> MNQNGDKNEGKLFQLPSLPPWKTPRFNKANFNNFTTPLRKRSTRVINDDSMPITGEVLEERTADDLYGINMDVDE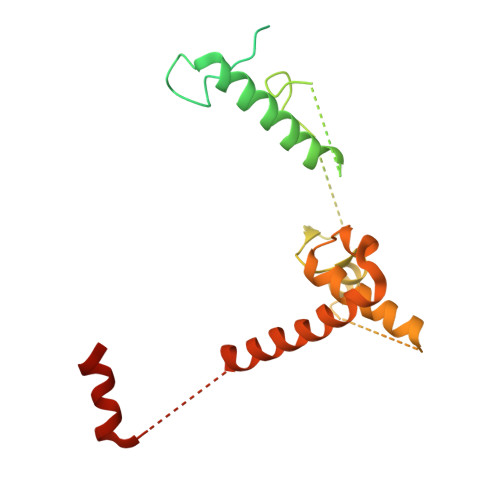VDYLNTLSHIEEEKQYDYSPFCERNTLRESRIDSFLKAERAAHCLVFHKVGHLDGIDSYRPDIDIMCGEEANKYDSANPEGNGSMLLESVPGCNKEDLERLSRREFVTNSKPNMRRLDDIINHETNALKSFWNDSGLVNSLQSHHLHEEYLLLQEELKNVYKIKCHDRVPIESLRDKCRRHYSNEDSSFL>MTATATEGAKPPFVSRSVLVTGGNRGIGLAIAQRLAADGHKVAVTHRGSGAPKGLFGVECDVTDSDAVDRAFTAVEEHQGPVEVLVSNAGLSADAFLMRMTEEKFEKVINANLTGAFRVAQRASRSMQRNKFGRMIFIGSVSGSWGIGNQANYAASKAG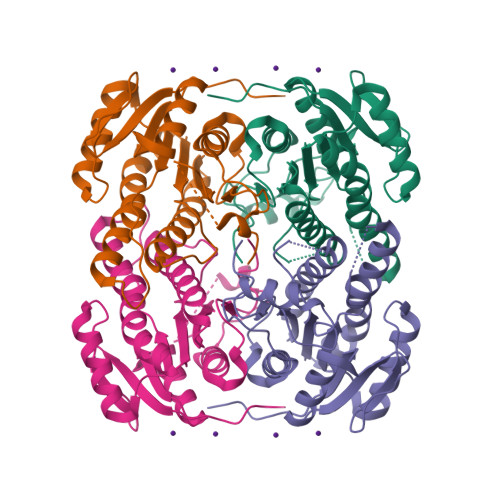VIGMARSIARELSKANVTANVVAPGYIDTDMTRALDERIQQGALQFIPAKRVGTPAEVAGVVSFLASEDASYISGAVIPVDGGMGMGH[2x]>SVKLAGNSSLCPVSGWAIYSKDNSVRIGSKGDVFVIREPFISCSPLECRTFFLTQGALLNDKHSNGTIKDRSPYRTLMSCPIGEVPSPYNSRFESVAWSASACHDGINWLTIGISGPDNGAVAVLKYNGIITDTIKSWRNNVLRTQESECACVNGSCFTVMTDGPSNGQASYKIFRIEKGKIVKSVEMNAPNYYYEECSCYPDSSEITCVCRDNWHGSNRPWVSFNQNLEYQIGYICSGIFGDNPRPNDKTGSCGPVSSNGANGVKGFSFKYGNGVWIGRTKSISSRNGFEMIWDPNGWTGTDNNFSIKQDIVGINEWSGYSGSFVQHPELTGLDCIRPCFWVELIRGRPKENTIWTSGSSISFCGVNSDTVGWSWPDGAELPFTIDK[4x]

NA is a homotetrameric transmembrane glycoprotein responsible for cleavage of sialic acid from the host cell membrane. By blocking NA enzymatic activity, neuraminidase inhibitors (NAIs) prevent new viral particles from being released from the surface of an infected cell, thus stopping the spread of virus in the airways. In this study, we applied a set of experimental techniques using recombinant NA variants to understand the molecular basis of development of oseltamivir resistance in the viral N1 neuraminidase NA2009. To decipher the structural mechanism of resistance, we determined crystal structures of NA2009 mutants in complex with oseltamivir carboxylate.

Three variants (H275Y, H275Y/I223V, and H275Y/S247N NA2009) crystallized in the monoclinic space group with four molecules in the asymmetric unit, representing the tetrameric biological unit. In enzyme variants containing H275Y in combination with the I223V or S247N mutation, an oseltamivir pose similar to that found in H275Y was observed. The RMSD for superposition of oseltamivir atoms in the H275Y, H275Y/I223V, and H275Y/S247N NA2009 variant was below 0.11 Å. We conclude that structural changes caused by the individual mutations have a coacting effect on increase of oseltamivir resistance, reflected in the more than three-fold increase in Ki in H275Y/I223V NA2009 compared to H275Y NA2009. The double mutations I223V/H275Y and S247N/H275Y led to dramatic increases in Ki values (3900- and 9000-fold higher than wt, respectively). We observed only moderately decreased catalytic efficiency (kcat/Km) for the single mutants I223V and S247N, and much lower values for all variants containing the H275Y substitution (only 4–6% of the wt value for the H275Y, I223V/H275Y, and S247N/H275Y mutants). The decrease in sensitivity to oseltamivir conferred by these single mutations alone is moderate, but when combined with the H275Y mutation, the double mutants have a greatly enhanced oseltamivir-resistant phenotype (1733-fold for H275Y/I223V and 7000-fold for H275Y/S247N compared to the recombinant wt virus).> PIQIGDLEIVPDAYVAKKYGEELDLTHREFELLYHLASHTGQVITREHLLETVWGYDYFGDVRTVDVTVRRLREKIEDTPSRPEYILTRRGVGYYMR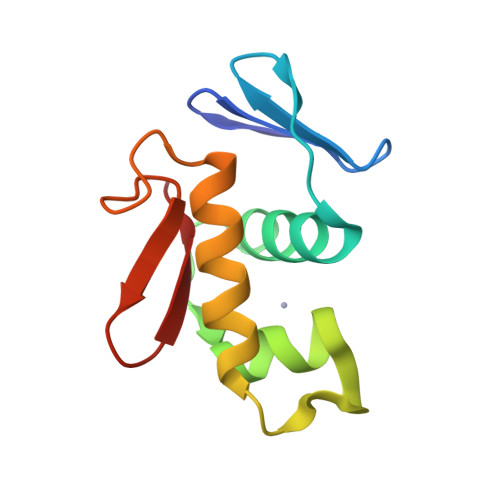N>GSHMLEMGDNLLQRIRLVVPSALQCCDGDLPIFDPQRPPARCVFQFNGEDNVSEAFPVEYIMRLMANWAQVDCDPYIKIQNTGVSVLFQGFFFRPTNAPVAEVSIDSNNVILSSTLSTGINLSALESIKRGGGIDRRPLQALMWVNCFVRMPYVQLSFRFMGPEDPSRTIKLMARATDAYMGGSGSGGSSKERSVYRHYFNYIARSPPEELATVRGLIVPIIKTTPVTLPFNLGQTVADNCLSLSGMGYHLGLGGYCPTCTASGEPRLCRTDRAALILAYVQQLNNIYEYRVFLASILALSDRANMQAASAEPLLSSVLAQPELFFMYHIMREGGMRDIRVLFYRDGDAGGFMMYVIFPGKSVHLHYRLIDHIQAACRGYKIVAHVWQTTFLLSVCRNPEQQTETVVPSIGTSDVYCKMCDLNFDGELLLEYKRLYAL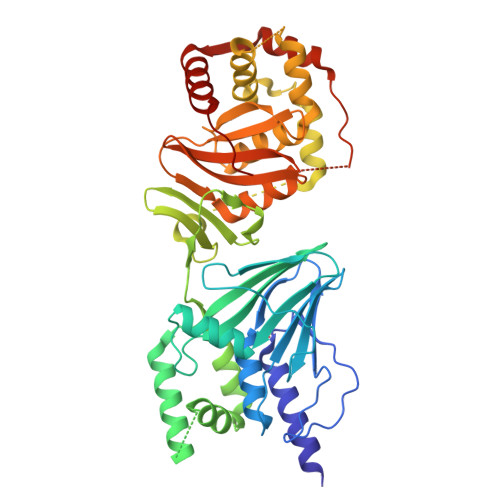FDDFVPPR[2x]> MHHHHHHSSGRENLYFQGTFAERYNIVCMLGKGSFGEVLKCKDRITQQEYAVKVINKASAKNKDTSTILREVELLKKLDHPNIMKLFEILEDSSSFYIVGELYTGGELFDEIIKRKRFSEHDAARIIKQVFSGITYMHKHNIVHRDLKPENILLESKEKDCDIKIIDFGLSTCFQQNTKMKDRIGTAYYIAPEVLRGTYDEKCDVWSAGVILYILLSGTPPFYGKNEYDILKRVETGKYAFDLPQWRTISDDAKDLIRKMLTFHPSLRITATQCLEHPWIQKYSSEE

In an endeavour to address the void, our study spans the classification of the C. parvum kinome and the structural and biochemical characterization of representatives from the CDPK family and a MAP kinase. Like in plants and ciliates, the CDPK family dominates the apicomplexan CaMK group. Many of the C. parvum CDPK enzymes have already been identified including: CpCDPK1 (cgd3_920), CpCDPK2 (cgd7_1840), CpCDPK2A (cgd2_1060), CpCDPK3 (cgd5_820), CpCDPK4 (cgd7_40), CpCDPK5 (cgd2_1300), and CpCDPK6 (cgd4_3330). For some time it has been known that the CDPK enzymes control crucial functions including transcription, metabolism, ion pumps and channels, and the cytoskeleton.

Inhibition of CpCDPK1 was thoroughly investigated by screening with a series of compounds designed to exploit the small gatekeeper that is naturally occurring in CpCDPK1, but not in the other CpCDPKs. For example, similar to previous results, pyrazolopyrimidine derivatives are ineffective against kinases with bulky gatekeepers (found just downstream of the catalytic lysine in a Yoo*xooxGGELFxxI motif, where o is hydrophobic, x is any, and * is the gatekeeper), but CpCDPK1 is expected to be sensitive to such inhibitors owing to the presence of a glycine instead of the typical methionine present in the remaining CpCDPKs. Accordingly, over a dozen PP1 derivatives were found that inhibit CpCDPK1 with IC50's less than 10 nM. The activation loop, which moves closer to the active site in the 3MB-PP1 structure sits lower and retains an additional turn at the top of the α-helix G in the apo structure. The pyrazolo-pyrimidine in the PP1 molecule occupies the same space where the adenine in ATP is typically found, forming H-bonds with the backbone of Glu153 and Tyr155. N8 of the 3MB-PP1 is linked by a water to the activating Lys105. The large, hydrophobic methylbenzyl group of 3MB-PP1 sits deep within the pocket lined by Leu222, Leu138, Ile150, and Met136. In most other kinases, this pocket is ablated by the side-chain of a large gatekeeper residue. The exploitation of the gatekeeper in the ATP-binding site shows that opportunities exist for inhibitor design, as is the case for CpCDPK1 which has a glycine-gatekeeper and is inhibited in the nanomolar range by PP1-derivatives. Indeed, our crystal structure highlights how one of these inhibitors functions.>[2x]MKSLGRHLVAEFYECDREVLDNVQLIEQEMKQAAYESGATIVTSTFHRFLPYGVSGVVVISEAHLTIHTWPEYGYAAI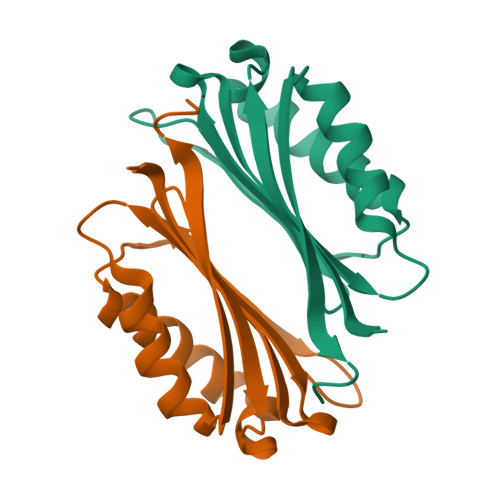DLFTCGEDVDPWKAFEHLKKALKAKRVHVVEHERGRYDEIGIPEDSPHKAAV> GSHMKLYIIGAGPGDPDLITVKGLKLLQQADVVLYADSLVSQDLIAKSKPGAEVLKTAGMHLEEMVGTMLDRMREGKMVVRVH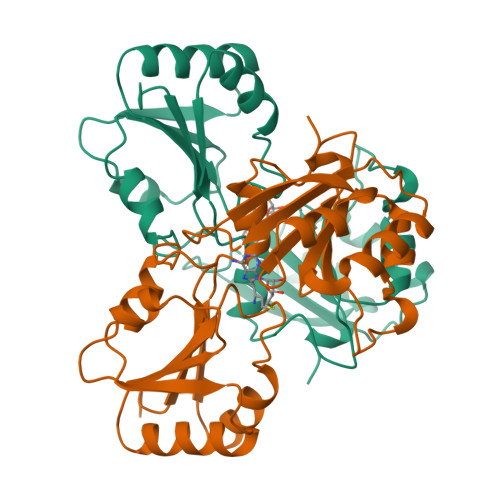TGDPAMYGAIMEQMVLLKREGVDIEIVPGVTSVFAAAAAAEAELTIPDLTQTVILTRAEGRTPVPEFEKLTDLAKHKCTIALFLSSTLTKKVMKEFINAGWSEDTPVVVVYKATWPDEKIVRTTVKDLDDAMRTNGIRKQAMILAGWALDP> MKLRMSRQDIRDEFKESEGDPHVKGKIRQMQRAAAQRRMMEDVPKADVIVTN;>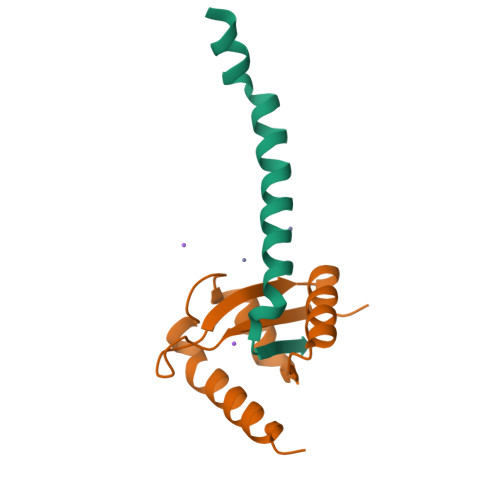 PTHYSVALQYDENKMSAPKVVAKGAGLIALRIREIGAEHRVPTLEAPPLARALYRHAEIGQQIPGQLYAAVAEVLAWVWQLKRWRLAGGQRPPQPENLPVPEALDFMNEKNTDA>MIIYRDLISHDEMFSDIYKIREIADGLCLEVEGKMVSRTEGNIDDSLIGGNASAEGPEGEGTESTVITGVDIVMNHHLQETSFTKEAYKKYIKDYMKSIKGKLEEQRPERVKPFMTGAAEQIKHILANFKNYQFFIGENMNPDGMVALLDYREDGVTPYMIFFKDGLEMEKC[4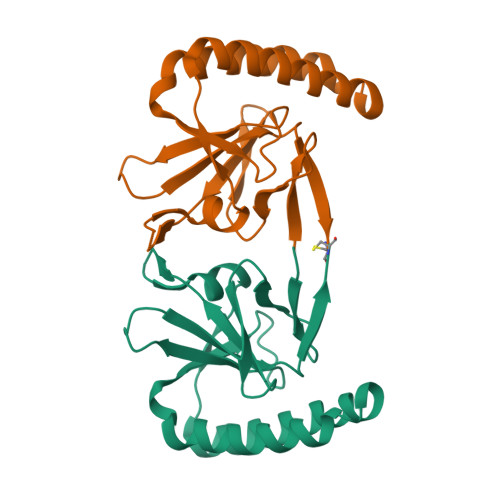x]> MDYQEYQQFLARINTARDACVAKDIDVDLLMARHDYFGRELCKSLNIEYRNDVPFIDIILDIRPEVDPLTIDAPHITPDNYLYINNVLYIIDYKVSVSNESSVITYDKYYELTRDISDRLSIPIEIVIIRIDPVSRDLHINSDRFKELYPTIVVDINFNQFFDLKQLLYEKFGDDEEFLLKVAHGDFTLTAPWCKTGCPEFWKHPIYKEFKMSMPVPERRLFEESVKFNAYESERWNTNLVKIREYTKKDYSEHISKSAKNIFLASGFYKQPNKNEISEGWTLMVERVQDQREISKSLHDQKPSIHFIWGAHNPGNSNNATFKLILLSKSLQSIKGISTYTEAFKSLGKMMDIGDKAIEYEEFCMSLKSKARSSWKQIMNKKLEPKQINNALVLWEQQFMINNDLIDKSEKLKLFKNFCGIGKHKQFKNKMLEDLEVSKPKILDFDDANMYLASLTMMEQSKKILSKSNGLKPDNFILNEFGSRIKDANKETYDNMHKIFETGYWQCISDFSTLMKNILSVSQYNRHNTFRIAMCANNNVFAIVFPSADIKTKKATVVYSIIVLHKEEENIFNPGCLHGTFKCMNGYISISRAIRLDKERCQRIVSSPGLFLTTCLLFKHDNPTLVMSDIMNFSIYTSLSITKSVLSLTEPARYMIMNSLAISSNVKDYIAEKFSPYTKTLFSVYMTRLIKNACFDAYDQRQRVQLRDIYLSDYDITQKGIKDNRELTSIWFPGSVTLKEYLTQIYLPFYFNAKGLHEKHHVMVDLAKTILEIECEQRENIKEIWSTNCTKQTVNLKILIHSLCKNLLADTSRHNHLRNRIENRNNFRRSITTISTFTSSKSCLKIGDFRKEKELQSVKQKKILEVQSRKMRLANPMFVTDEQVCLEVGHCNYEMLRNAMPNYTDYISTKVFDRLYELLDKKVLTDKPVIEQIMDMMIDHKKFYFTFFNKGQKTSKDREIFVGEYEAKMCMYAVERIAKERCKLNPDEMISEPGDGKLKVLEQKSEQEIRFLVETTRQKNREIDEAIEALATEGYESNLGKIEKLSLGKAKGLKMEINADMSKWSAQDVFYKYFWLIALDPILYPQEKERILYFMCNYMDKELILPDELLFNLLDQKVAYQNDIIATMTNQLNSNTVLIKRNWLQGNFNYTSSYVHSCAMSVYKEILKEAITLLDGSILVNSLVHSDDNQTSITIVQDKMENDKIIDFAMKEFERACLTFGCQANMKKTYVTNCIKEFVSLFNLYGEPFSIYGRFLLTSVGDCAYIGPYEDLASRISSAQTAIKHGCPPSLAWVSIAISHWMTSLTYNMLPGQSNDPIDYFPAENRKDIPIELNGVLDAPLSMISTVGLESGNLYFLIKLLSKYTPVMQKRESVVNQIAEVKNWKVEDLTDNEIFRLKILRYLVLDAEMDPSDIMGETSDMRGRSILTPRKFTTAGSLRKLYSFSKYQDRLSSPGGMVELFTYLLEKPELLVTKGEDMKDYMESVIFRYNSKRFKESLSIQNPAQLFIEQILFSHKPVIDFSGIRDKYINLHDSRALEKEPDILGKVTFTEAYRLLMRDLSSLELTNDDIQVIYSYIILNDPMMITIANTHILSIYGSPQRRMGMSCSTMPEFRNLKLIHHSPALVLRAYSKNNPDIQGADPTEMARDLVHLKEFVENTNLEEKMKVRIAMNEAEKGQRDIVFELKEMTRFYQVCYEYVKSTEHKIKVFILPAKSYTTTDFCSLMQGNLIKDKEWYTVHYLKQILSGGHKAIMQHNATSEQNIAFECFKLITHFADSFIDSLSRSAFLQLIIDEFSYKDVKVSKLYDIIKNGYNRTDFIPLLFRTGDLRQADLDKYDAMKSHERVTWNDWQTSRHLDMGSINLTITGYNRSITIIGEDNKLTYAELCLTRKTPENITIS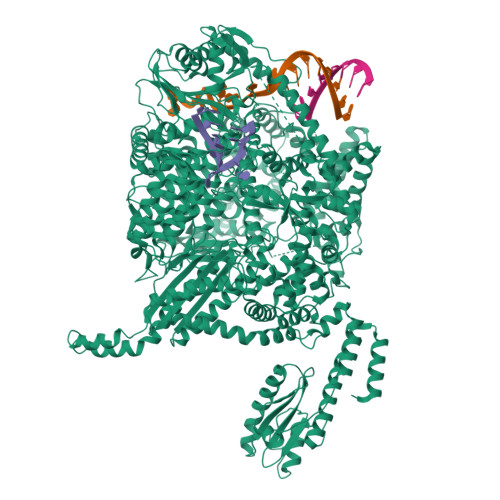GRKLLGSRHGLKFENMSKIQTYPGNYYITYRKKDRHQFVYQIHSHESITRRNEEHMAIRTRIYNEITPVCVVNVAEVDGDQRILIRSLDYLNNDIFSLSRIKVGLDEFATIKKAHFSKMVSFEGPPIKTGLLDLTELMKSQDLLNLNYDNIRNSNLISFSKLICCEGSDNINDGLEFLSDDPMNFTEGEAIHSTPIFNIYYSKRGERHMTYRNAIKLLIERETKIFEEAFTFSENGFISPENLGCLEAVVSLIKLLKTNEWSTVIDKCIHICLIKNGMDHMYHSFDVPKCFMGNPITRDINWVMFREFINSLPGTDIPPWNVMTENFKKKCIALINSKFETQRDFSEFTKLMKKEGGRSNIEFD> GMENFIGSHMIYTYENGWEYEIYIKNDHTIDYRIHSGMVAGRWVRDQEVNIVKLTEGVYKVSWTEPTGTDVSLNFMPNEKRMHGIIFF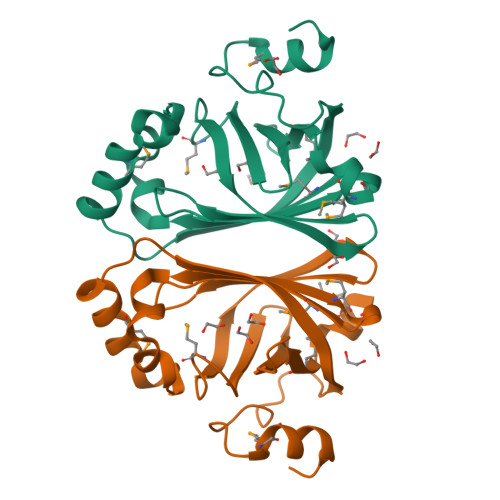PKWVHEHPEITVCYQNDHIDLMKESREKYETYPKYVVPEFAEITFLKNEGVDNEEVISYAPYEGMTDDIRAGRL>[3x]MSIVFASIDPRSNPLQTSSQNYVDIPGLKLDVSKYSNSPCLTALITLNI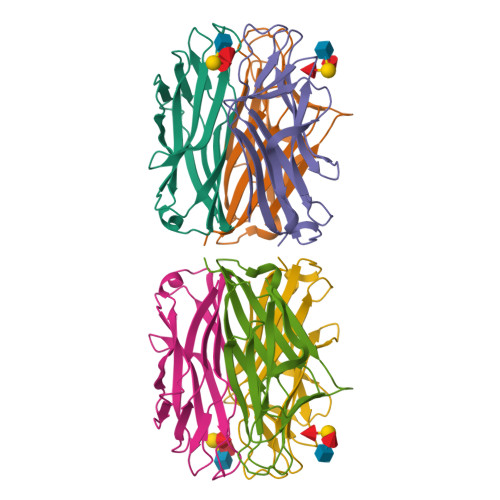PTPYASGNNFPGGNFAIVTDQGEQLAYGGFTYSSKIPENSGRMPFTLVARYSLASNVSTIKAQWSNIRGSTVHIDSYASISAVIQCNQLV>MGSHHHHHHDITSLYKKAGSAAAVLEENLYFQGSFTMLHEIPKSEILKELKRIGAKRVLIQSPEGLRREAEELAGFLEENNIEVFLHGEINYGACDPADREAKLVGCDALIHLGHSYMKLPLEVPTIFVPAFARVSVVEALKENIGEIKKLGRKIIVTTTAQHIHQLKEAKEFLESEGFEVSIGRGDSRISWPGQVLGCNYSVAKVRGEGILFIGS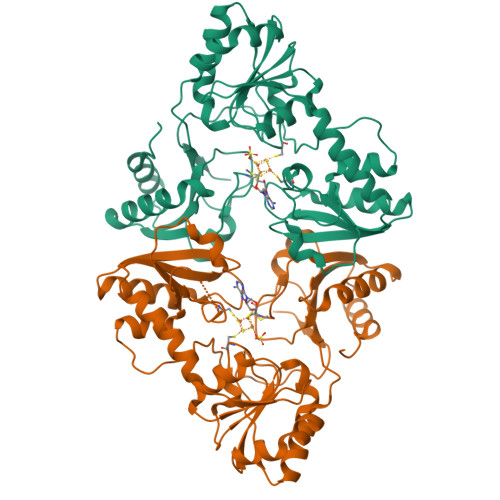GIFHPLGLAVATRKKVLAIDPYTKAFSWIDPERFIRKRWAQIAKAMDAKKFGVIVSIKKGQLRLAEAKRIVKLLKKHGREARLIVMNDVNYHKLEGFPFEAYVVVACPRVPLDDYGAWRKPVLTPKEVEILLGLREEYEFDEILGGPRESDEPFGISIHSTR[2x]> SGRPMTYADYFSAWDKWEKQALPGEERDEAVSRLKECLINNSDELRLDRLNLSSLPDNLPAQITLLNVSYNQLTNLPELPVTLKKLYSASNKLSELPVLPPALESLQVQHNELEN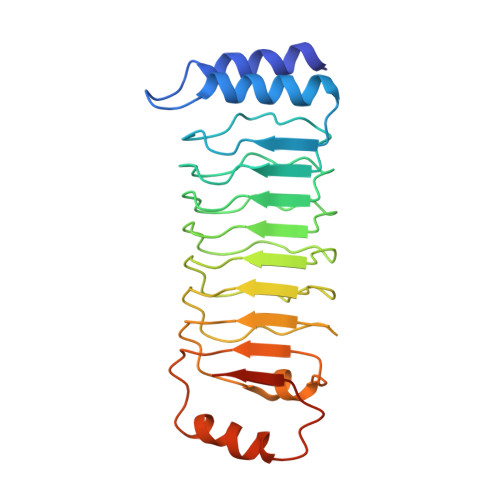LPALPDSLLTMNISYNEIVSLPSLPQALKNLRATRNFLTELPAFSEGNNPVVREYFFDRNQISHIPESILNLRNECSIHISDNPLSSHALPALQRLTSSPDYHGPRIYFSMSDGQQNTLHR> SRLDPDPEFIGFINNVTYPA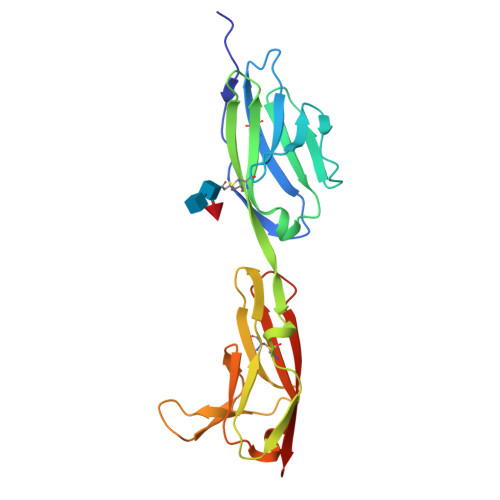GREAILACSVRNLGKNKVGWLRASDQTVLALQGRVVTHNARISVMHQDMHTWKLKISKLRESDRGCYMCQINTSPMKKQVGCIDVQVPPDIINEESSADLAVQEGEDATLTCKATGNPQPRVTWRREDGEMILIRKPGSRELMKVESYNGSSLRLLRLERRQMGAYLCIASNDVPPAVSKRVSLSVHHHHHHH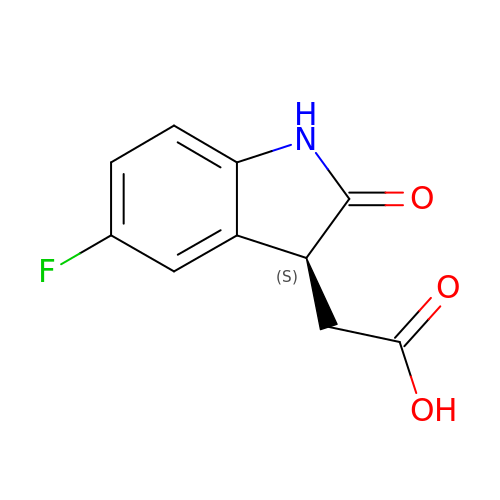2-[(3S)-5-fluoranyl-2-oxidanylidene-1,3-dihydroindol-3-yl]ethanoic acid | C10 H8 F N O3 | GOJAJUSLXBXIJY-ZETCQYMHSA-N>MGHHHHHHHHHHMQSSVNEFLTPRHIDVQVVSQTRAKITLEPLERGFGHTLGNALRRILLSSMPGCAVVEAEIDGVLHEYSAIEGVQEDVIEILLNLKGLAIKLHGRDEVTLTLAKKGSGVVTAADIQLDHDVEIINGDHVIANLADNGALNMKLKVARGRGYEPADARQSDEDESRSIGRLQLDASFSPVRRVSYVVENARVEQRTNLDKLVLDLETNGTLDPEEAIRRAATILQQQLAAFVDLKGDSEPVVEEQEDEIDPILLRPVDDLELTVRSANCLKAENIYYIGDLIQRTEVELLKTPNLGKKSLTEIKDVLASRGLSLGMRLDNWPPASLKKDDKATA[2x];> MGMAYSYTEKKRIRKDFSKLPDVMDVPYLLAIQLDSYREFLQAGATKEQFRDVGLHAAFKSVFPIISYSGNAALEYVGYRLGEPAFDVKECVLRGVTFAVPLRVKVRLIIFDRESSNKAIKDIKEQEVYMGEIPLMTENGTFIINGTERVIVSQLHRSPGVFFDHDRGKTHSSGKLLYSARIIPYRGSWLDFEFDPKDCVFVRIDRRRKLPASVLLRALGYSTEEILNAFYATNVFHIKGETLNLELVPQRLRGEVASIDIKDGSGKVIVEQGRRITARHINQLEKAGVSQLEVPFDYLIGRTIAKAIVHPATGEIIAECNTELTLDLLAKVAKAQVVRIETLYTNDIDCGPFISDTLKIDNTSNQLEALVEIYRMMRPGEPPTKEAAETLFGNLFFSAERYDLSAVGRMKFNRRIGRTEIEGPGVLSKEDIIDVLKTLVDIRNGKGIVDDIDHLGNRRVRCVGEMAENQFRVGLVRVERAVKERLSMAESEGLMPQDLINAKPVAAAIKEFFGSSQLSQFMDQNNPLSEITHKRRVSALGPGGLTRERAGFEVRDVHPTHYGRVCPIETPEGPNIGLINSLATYARTNKYGFLESPYRVVKDSLVTDEIVFLSAIEEADHVIAQASATLNEKGQLVDELVAVRHLNEFTVKAPEDVTLMDVSPKQVVSVAASLIPFLEHDDANRALMGSNMQRQAVPTLRADKPLVGTGMERNVARDSGVCVVARRGGVIDSVDASRVVVRVADDEVETGEAGVDIYNLTKYTRSNQNTCINQRPLVSKGDVVARGDILADGPSTDMGELALGQNMRVAFMPWNGFNFEDSICLSERVVQEDRFTTIHIQELTCVARDTKLGPEEITADIPNVGEAALNKLDEAGIVYVGAEVQAGDILVGKVTPKGETQLTPEEKLLRAIFGEKASDVKDTSLRVPTGTKGTVIDVQVFTRDGVERDSRALSIEKMQLDQIRKDLNEEFRIVEGATFERLRAALVGAKAEGGPALKKGTEITDDYLDGLERGQWFKLRMADDALNEQLEKAQAYISDRRQLLDDKFEDKKRKLQQGDDLAPGVLKIVKVYLAIKRRIQPGDKMAGRHGNKGVVSVIMPVEDMPHDANGTPVDIVLNPLGVPSRMNVGQILETHLGLAAKGLGEKINRMLEEQRKVAELRKFLHEIYNEIGGREENLDELGDNEILALAKNLRGGVPMATPVFDGAKEREIKAMLKLADLPESGQMRLFDGRTGNQFERPTTVGYMYMLKLNHLVDDKMHARSTGSYSLVTQQPLGGKAQFGGQRFGEMEVWALEAYGAAYTLQEMLTVKSDDVNGRTKMYKNIVDGDHRMEAGMPESFNVLIKEIRSLGIDIELETE;> MLKDLLNLLKNQGQIEEFDAIRIGLASPEMIRSWSFGEVKKPETINYRTFKPERDGLFCAKIFGPVKDYECLCGKYKRLKHRGVICEKCGVEVALAKVRRERMGHIELASPVAHIWFLKSLPSRIGLLLDMTLRDIERVLYFESYVVIDPGMTTLEKGQLLNDEQYFEALEEFGDDFDARMGAEAVHELLNAIDLEHEIGRLREEIPQTNSETKIKKLSKRLKLMEAFQGSGNKPEWMVLTVLPVLPPDLRPLVPLDGGRFATSDLNDLYRRVINRNNRLKRLLDLAAPDIIVRNEKRMLQEAVDALLDNGRRGRAITGSNKRPLKSLADMIKGKQGRFRQNLLGKRVDYSGRSVITVGPTLRLHQCGLPKKMALELFKPFIFGKLEGRGMATTIKAAKKMVERELPEVWDVLAEVIREHPVLLNRAPTLHRLGIQAFEPVLIEGKAIQLHPLVCAAYNADFDGDQMAVHVPLTLEAQLEARALMMSTNNILSPANGEPIIVPSQDVVMGLYYMTREAINAKGEGMAFADLQEVDRAYRSGQASLHARVKVRINEKIKGEDGQLTANTRIVDTTVGRALLFQVVPAGLPFDVVNQSMKKKAISKLINHCYRVVGLKDTVIFADQLMYTGFAYSTISGVSIGVNDFVIPDEKARIINAATDEVKEIESQYASGLVTQGEKYNKVIDLWSKANDEVSKAMMANLSKEKVVDREGKEVDQESFNSMYMMADSGARGSAAQIRQLAGMRGLMAKPDGSIIETPITANFREGLNVLQYFISTHGARKGLADTALKTANSGYLTRRLVDVAQDLVVTEIDCGTEHGLLMSPHIEGGDVVEPLGERVLGRVIARDVFKPGSDEVIVPAGTLIDEKWVDFLEVMSVDEVVVRSPITCETRHGICAMCYGRDLARGHRVNIGEAVGVIAAQSIGEPGTQLTMRTFHIGGAASRTSAADNVQVKNGGTIRLHNLKHVVRADGALVAVSRSGELAVADDFGRERERYKLPYGAVISVKEGDKVDPGAIVAKWDPHTHPIVTEVDGTVAFVGMEEGITVKRQTDELTGLTNIEVMDPKDRPAAGKDIRPAVKLIDAAGKDLLLPGTDVPAQYFLPANALVNLTDGAKVSIGDVVARIPQETSKTRDITGGLPRVADLFEARRPKEPSILAEISGTISFGKETKGKRRLVITPNDGSDPYEELIPKWRHLNVFEGEQVNRGEVISDGPSNPHDILRLLGVSSLAKYIVNEIQDVYRLQGVKINDKHIETILRQMLRKVEVSESGDSSFIKGDQVELTQVLEENEQLGTEDKFPAKYERVLLGITKASLSTESFISAASFQETTRVLTEAAVTGKRDFLRGLKENVVVGRLIPAGTGLAYHSERKRQRDLGKPQRVSASEAEAALTEALNSSGNGSGSWSHPQFEK;> MARVTVEDCLDNVDNRFELVMLATKRARQLATGGKEPKVAWENDKPTVVALREIASGLVDENVVQQEDIVEDEPLFAAFDDEANTEAL;> GAMGMALKKEGPEFDHDDEVLLLEPGIMLDESSADEQPSPRATPKATTSFSSKQHKHIDYTRALDATQLYLNEIGFSPLLTPEEEVHFARLAQKGDPAGRKRMIESNLRLVVKIARRYVNRGLSLLDLIEEGNLGLIRAVEKFDPERGFRFSTYATWWIRQTIERAIMNQTRTIRLPIHVVKELNVYLRAARELTHKLDHEPSPEEIANLLEKPVAEVKRMLGLNERVTSVDVSLGPDSDKTLLDTLTDDRPTDPCELLQDDDLSESIDQWLTELTDKQREVVIRRFGLRGHESSTLEEVGQEIGLTRERVRQIQVEALKRLREILEKNGLSSDALFQ;> GAMGMSEEELEQDELDGADEDDGEELAAADDGEADSGDGDEAPAPGKKAKAAVVEEELPSVEAKQKERDALAKAMEEFLSRGGKVQEIEPNVVADPPKKPDSKYGSRPI

Pseudomonas aeruginosa (Pae) SutA adapts bacteria to hypoxia and nutrition-limited environment during chronic infection by increasing transcription activity of an RNA polymerase (RNAP) holoenzyme comprising the stress-responsive σ factor σS (RNAP-σS). To understand the molecular mechanism of SutA activation, here we determined cryo-EM structures of RNAP-σS holoenzyme at 4.1 Å, SutA-bound RNAP-σS holoenzyme at 3.1 Å (SutA-RNAP-σS, open lobe) and 3.9 Å (SutA-RNAP-σS, closed lobe), and SutA-bound RNAP-σS promoter open complex (SutA-σS-RPo) at 5.8 Å. The structures reveal that SutA pinches RNAP-β protrusion with its RNAP-binding domain and wedges RNAP-β lobe open to facilitate promoter unwinding with its wedge loop and N-terminal D/E-rich region. SutA anchors RNAP-β protrusion through its RBD and wedges open β lobe through its wedge loop to facilitate RPo formation.

Focused 3D classification reveals one major population of SutA-bound RNAP-σS single particles, from which a cryo-EM map was reconstructed at a resolution of 3.1 Å, and one minor population of SutA-bound RNAP-σS single particles, from which a cryo-EM map was reconstructed at a resolution of 3.9 Å. In the structure of SutA-RNAP-σS (open lobe), the RNAP-β protrusion is embraced by a patch of crescent-shaped map that could be assigned to SutA-RBD, consistent with our YTH results and cross-linking data in a previous study. The 3.1 Å cryo-EM map exhibits clear feature of an α-helix in the middle of the crescent-shaped map that fits well to the 20-residue predicted helical region (residues 57–76). One end of the crescent (residues 77-90) travels across the surface of the RNAP-β protrusion and approaches σ3.1, four residues (81–84) of which likely form a 4-strand β sheet with RNAP-β protrusion. The other end of the crescent (residues 54-57; wedge loop) fits into the narrow gap between RNAP-β protrusion and β lobe and leads the rest part of SutA-NTD to the main cleft, where it likely adopts an assemble of multiple conformations and thereby does not show distinct map signals. SutA-RBD occupies a hydrophobic groove on RNAP-β protrusion. Several hydrophobic residues of SutA (L67, M71, F74, L75, V81, and I84) likely participate in the interaction. In the SutA-RNAP-σS (open lobe) structure, the RNAP-β lobe domain swings ~10° away from RNAP-β’ clamp resulting in ~5 Å increase in distance between RNAP-β’ clamp and RNAP-β lobe compared with that of RNAP-σS holoenzyme. The gate loop (RNAP-β residues 373-383; corresponding to RNAP-β residues 368-378 in E. coli), which serves as a rate-limiting gate for promoter loading in E. coli and M. tuberculosis RNAP, is opened along with the movement of β lobe. The main cleft of SutA-RNAP-σS (open lobe) can accommodate the downstream dsDNA as shown by structural modelling.2-[(1R)-1-aminopropyl]phenol 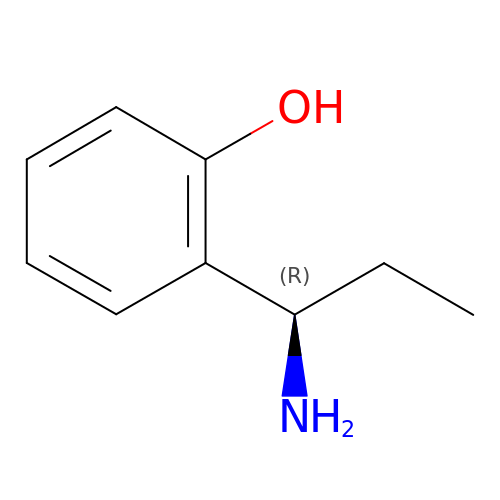| C9 H13 N O | SJYRIEHMQRIBEN-MRVPVSSYSA-N> LKESPSGYLRSGEGDTGCGELVWVGEPLTLRTAETITGKYGVWMRDPKPTYPYTQETTWRIDTVGTDVRQVFEYDLISQFMQGYPSKVHILPRPLESTGAVVYSGSLYFQGAESRTVIRYELNTEIVKAEKEIPGAGYHGQFPYSWGGYTDIDLAVDEAGLWVIYSTDEAKGAIVLSKLNPENLELEQTWETNIRKQSVANAFIICGTLYTVSSYTSADATVNFAYDTGTGISKTLTIPFKNRYKYSSMIDYNPLEKKLFAWDNLNMVTYDIKLSKM

Inherited missense mutations in the myocilin (MYOC) gene, within its olfactomedin (OLF) domain, constitute the strongest genetic link to primary open-angle glaucoma via a toxic gain of function, and thus MYOC is an attractive precision-medicine target. Myocilin has no known function, and there is no glaucoma phenotype in Myoc knockout mice or in individuals with a homozygous N-terminal truncation mutation or hemizygous deletion of MYOC, but rare non-synonymous coding mutations lead to toxic intracellular sequestration of misfolded myocilin. However, not all mutations in MYOC cause glaucoma, and common variants are expected to be neutral polymorphisms. Among the common features associated with pathogenic myocilin misfolding, we demonstrate that a single metric, OLF thermal stability, can robustly segregate benign from early-onset disease variants.

At the outset of our study, five variants could be confidently predicted as benign polymorphisms: T293K, T353I, K398R, A445V and K500R. These mutations are all found on the protein surface and well documented in the literature. Thr to Lys and Thr to Ile are less conservative changes, but in prior studies, T293K and T353I exhibited wild type (WT)-like cellular secretion and WT-like thermal stability, and were found in the control group for case–control clinical studies. Assessment of spent media from cells expressing each of the 16 full-length myocilin variants revealed WT-like secretion for T256M, R296H, L303I, S313F, V329M, S331L, T353I, A445V, V449I and K500R. The detergent-insoluble myocilin fractions were highest for E300K, S313F, T353I and N420Y. Indeed, in our cellular assay, some misfolding characteristics were initially detected for T353I and S313F but, ultimately, other characteristics including thermal stabilities were found to be within the bounds of benign variants. Structural integrity was further confirmed by high-resolution crystal structures, which were solved for 11 OLF variants. No gross changes from WT OLF were detected for the structures of T293K, R296H, L303I, V329M, S331L, E352K, T353I, K398R, A445V, V449I or K500R, indicating that these mutations are accommodated within the native five-bladed β-propeller fold and do not perturb the dinuclear calcium-containing site.> MSTENRVIDIVVDEKVPYGLIMQFMDVDDSVYPPSEIPVNLTGYSLRGT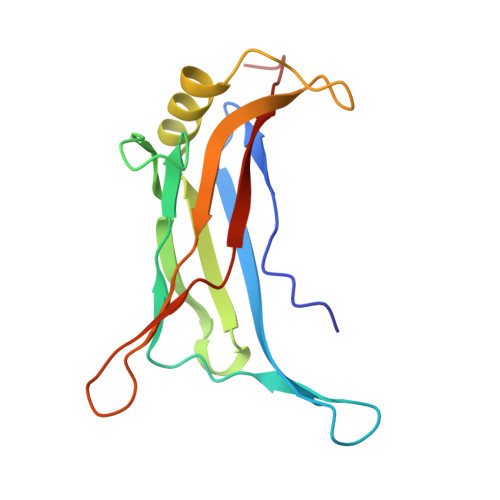IKSSLDENAETLASFTTSIIDAAQGAAAISLSVADVTNIGEKASKERDKYNPRQRFAGYYDILMTRDVIGSEVSSFRIMEGKVYISDGVTQ> MTTLTLSEAAPLLKKEFREGRLIPFLGAGFSKPLKLPDGSQLIASLAKTLGFEPELFDMHGRFEQLAEFFAISAPNRLQRLVYEMSLSFDSAEAEALREKSPMHRALAALDWRTIYTTNYDKHVEGALRDAGKQAAVLASFADFQGPRARDVCEVIKFHGTLDQPDTIVLTESSYFQRMALDAPPDQRLRADLLANSFLFIGYSFSDTNIRYIWYRMNQLREQSQLGVKHSQARRCFFATHGAGLVQ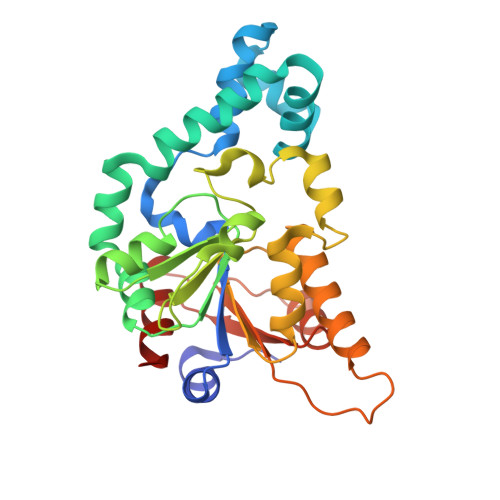PDILQQWNIDVIQLDPTDKSASVARLLESIA>[2x]ALEKVPVEEYLVHALQGSVSSGQAHSLASLAKTWSSGSAKLQRLGPETEDNEGVLLTEKLKPVDYEYREEVHWMTHQPRVGRGSFGEVHRMKDKQTGFQCAVKKVRLEVFRVEELVACAGLSSPRIVPLYGA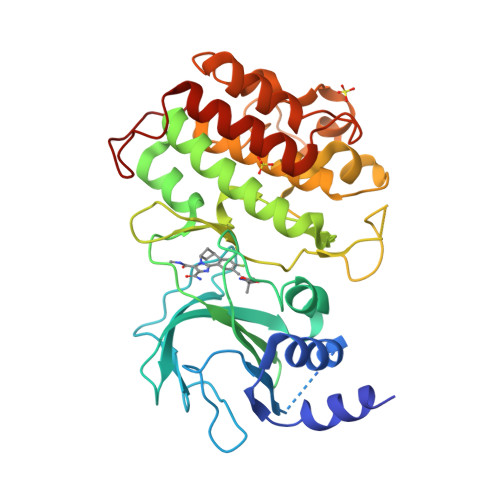VREGPWVNIFMELLEGGSLGQLIKQMGCLPEDRALYYLGQALEGLEYLHTRRILHGDVKADNVLLSSDGSRAALCDFGHALCLQPDGLGKSLLTGDYIPGTETHMAPEVVMGKPCDAKVDIWSSCCMMLHMLNGCHPWTQYFRGPLCLKIASEPPPIREIPPSCAPLTAQAIQEGLRKEPVHRASAMELRRKVGKALQEVGGLKSPWKGEYKEPR> LRPVLPTQSAHDPPAVHLSNGPGQEPIAVMTFDLTKITKTSSSFEVRTWDPEGVIFYGDTNPKDDWFMLGLRDGRPEIQLHNHWAQLTVGAGPRLDDGRWHQVEVKMEGDSVLLEVDGEEVLRLRQVSGPLTSKRHPIMRIALGGLLF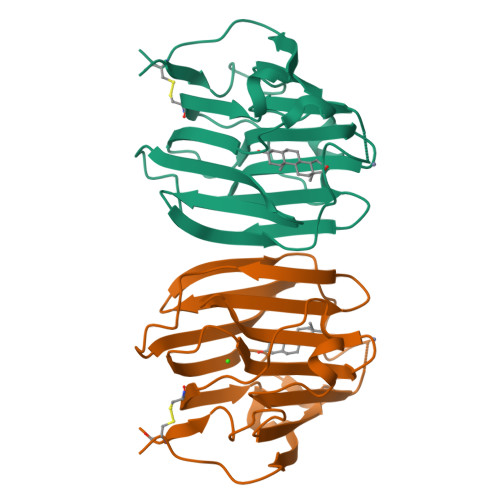PASNLRLPLVPALDGCLRRDSWLDKQAEISASAPTSLRSCD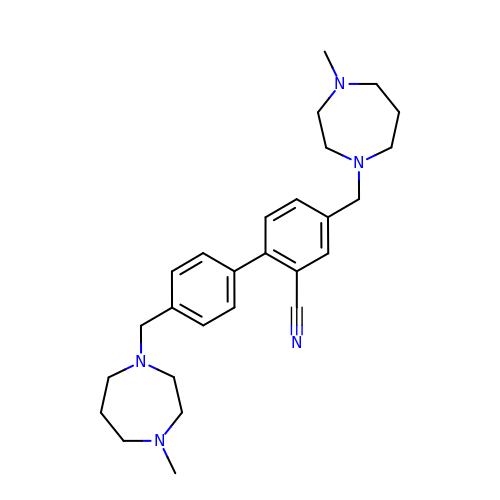5-[(4-methyl-1,4-diazepan-1-yl)methyl]-2-[4-[(4-methyl-1,4-diazepan-1-yl)methyl]phenyl]benzenecarbonitrile | C27 H37 N5 | MJTWJYMXCDQAOT-UHFFFAOYSA-N>[2x]TYTISIRVYQTTPKGFFRPVERTNWKYANGGTWDEVRGEYVLTMGGSGTSGSLRFVSSDTDESFVATFGVHNYKRWCDIVTNLTNEQTALVINQEYY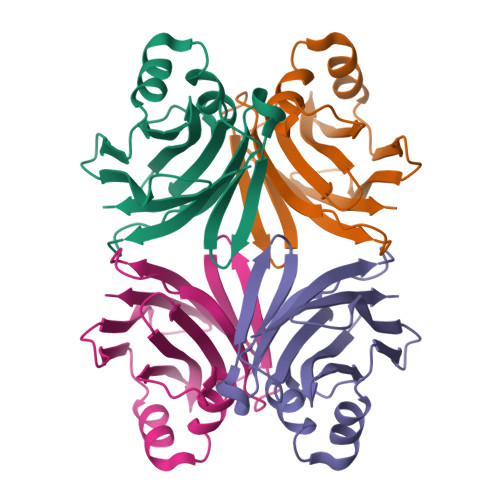GVPIRDQARENQLTSYNVANAKGRRFAIEYTVTEGDNLKANLIIG> UUUUUCAGUUAGAGCGUCGUGUCUCUUGUACGUCUCGGUCACAAUACACGGUUUCGUCCGGUGCGUGGCAAUUCGGGGCACAUCAUGUCUUUCGUGGCUGGUGUGACCG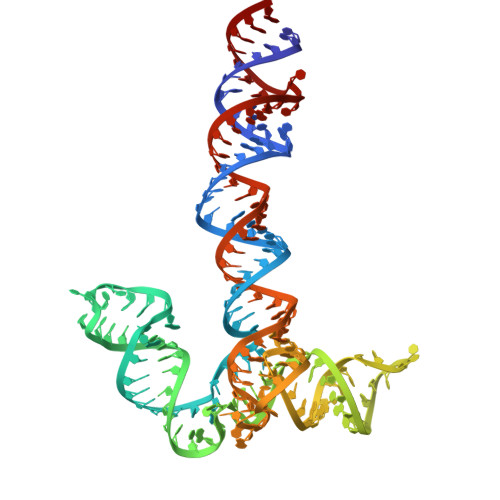CGCAAGGUGCGCGCGGUACGUAUCGAGCAGCGCUCAACUCUGAAAAA> NDFKNHQLPL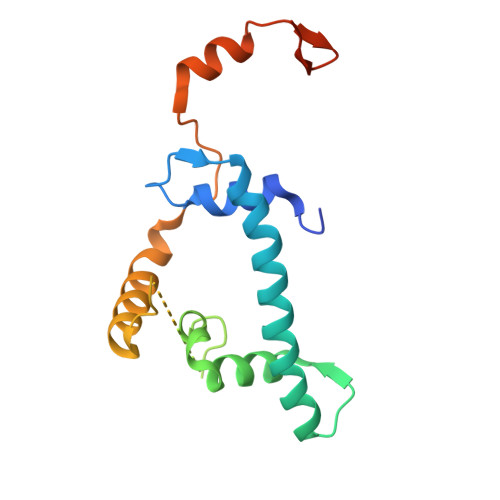ARIKKIMKADEDVRMISAEAPILFAKACELFILELTIRSWLHAEENKRRTLQKNDIAAAITRTDIFDFLVDIVPRGSGSGSGSGSGSDPASQMITVTQLSPMDREARVLRYREKRKTRKFEKTIRYASRKAYAEIRPRVNGRFAKREIEAEEQGF> MIERLNSPFLRAAALFTIVAFSSLISTAALAENNPSDTAKKFKVVTTFTIIQDIAQNIAGDVAVVESITKPGAEIHDYQPTPRDIVKAQSADLILWNGMNLERWFEKFFESIKDVPSAVVTAGITPLPIREGPYSGIANPHAWMSPSNALIYIENIRKALVEHDPAHAETYNRNAQAYAEKIKALDAPLRERLSRIPAEQRWLVTSEGAFSYLAKDYGFKEVYLWPINAEQQGIPQQVRHVIDIIRENKIPVVFSESTISDKPAKQVSKETGAQYGGVLYVDSLSGEKGPVPTYISLINMTVDTIAKGFGQ

Bacterial substrate-binding proteins (SBPs) belong to the widespread ABC superfamily and specifically have a role in sequestering various metabolites, including amino acids, nucleic acids, carbohydrates and metals. All SBPs follow an evolution­arily conserved c-clamp architecture containing α/β globular lobe domains connected by a backbone and interdomain β-strand hinges. Recently, we determined the crystal structure of holo YfeA, a Yersinia pestis polyspecific cluster A-I SBP, and reported a method for purifying apo YfeA in the presence of the Yfe transporter by fractionation, adding an additional strategy for the production of apo SBP proteins. In this report, we solved the crystal structure of apo YfeA as well as that of holo YfeA that was reconstituted by soaking crystals of apo YfeA with zinc.

A possible explanation for the improvement might be that gentle pipetting better preserved the sphero­plasts, reducing inadvertent rupture of the inner membrane and contamination of the periplasm with cytoplasmic contents, including metals that can reintegrate with a potentially apo YfeA. These changes enabled the purification and crystallization of seemingly apo YfeA protein exhibiting relatively low EDS signals [Fig. 1(a)]. Diffraction-quality apo native YfeA crystals were observed to crystallize in the orthorhombic space group P212121 and had unit-cell parameters a = 40, b = 52, c = 113 Å, which are 2 Å smaller in the a dimension than the unit-cell parameters of the His-tagged holo YfeA crystal form 1 (a = 42, b = 52, c = 113 Å; Radka, DeLucas et al., 2017). Apo YfeA contains 111 disordered protein atoms in a mobile helix and a 94.0 Å2 metal-binding site. The missing amino-acid residues constitute the base of the flexible helix 7 and the subsequent loop that have been proposed to undergo structural rearrangement during metal transfer. Close inspection of the changes in site 1 between the apo and the reconstituted holo forms identifies the key change that triggers the spontaneous refolding of the mobile helix in the flexible lobe and closure of the c-clamp. In the apo structure, the site 1 residue Glu207 is completely disengaged and a placeholder water molecule is observed to coordinate the nearby residue Glu256 and to establish tetrahedral coordination of a site 1 water molecule [Fig. 3(a)]. In this conformation, the site 1 residues His76, His141 and Asp282 remain grouped together as an electrostatic touch fastener primed to mate with a metal atom. In the apo state, YfeA has three grouped (His76/His141/Asp282) site 1 metal-binding residues linked to a rigid amino-terminal domain lobe that serve as an electrostatic attractant for metal ions. A fourth, disengaged site 1 residue (Glu207) is linked to a flexible carboxy-terminal domain lobe containing 111 disordered protein atoms from a mobile helix.>PFITVGQENSTSIDLYYEDHGAGQPVVLIHGFPLSGHSWERQSAALLDAGYRVITYDRRGFGQSSQPTTGYDYDTFAADLNTVLETLDLQDAVLVGFSMGTGEVARYVSSYGTARIAKVAFLASLEPFLLKTDDNPDGAAPKEFFDGIVAAVKADRYAFYTGFFNDFYNLDENLGTRISEEAVRNSWNTAASGGFFAAAAAPTTWYTDFRADIPRIDVPALILHGTGDRTLPIENTARVFH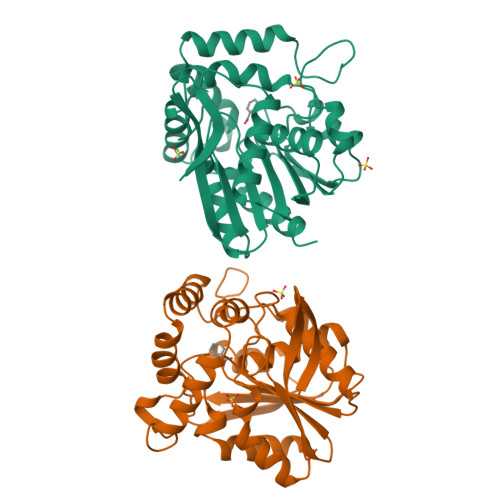KALPSAEYVEVEGAPHGLLWTHAEEVNTALLAFLAK[2x]ethyl 4-[(4-pyrazol-1-ylphenyl)methylcarbamoylamino]benzoate | 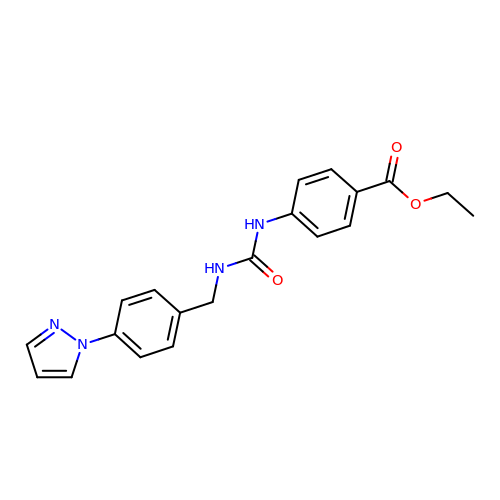C20 H20 N4 O3 | KQUKHINHCUELQL-UHFFFAOYSA-N> MRGSHHHHHHGSRVMVIGGDGYC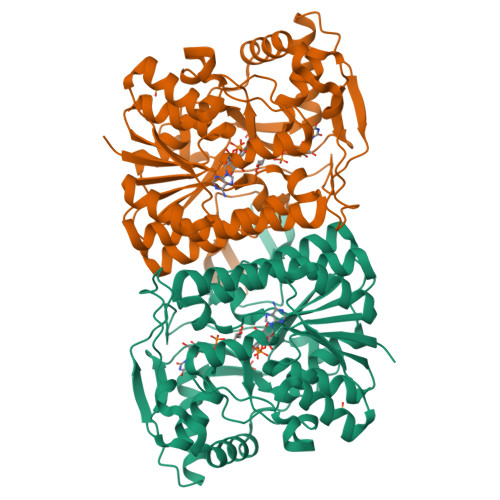GWATALHLSKKNYEVCIVDNLVRRLFDHQLGLESLTPIASIHDRISRWKALTGKSIELYVGDICDFEFLAESFKSFEPDSVVHFGEQRSAPYSMIDRSRAVYTQHNNVIGTLNVLFAIKEFGEECHLVKLGTMGEYGTPNIDIEEGYITITHNGRTDTLPYPKQASSFYHLSKVHDSHNIAFTCKAWGIRATDLNQGVVYGVKTDETEMHEELRNRLDYDAVFGTALNRFCVQAAVGHPLTVYGKGGQTRGYLDIRDTVQCVEIAIANPAKAGEFRVFNQFTEQFSVNELASLVTKAGSKLGLDVKKMTVPNPRVEAEEHYYNAKHTKLMELGLEPHYLSDSLLDSLLNFAVQFKDRVDTKQIMPSVSWKKIGVKTKSMTT> SMIDDDGYRPNVGIVICNRQGQVMWARRFGQHSWQFPQGGINPGESAEQAMYRELFEEVGLSRKDVRILASTRNWLRYKLPKRLV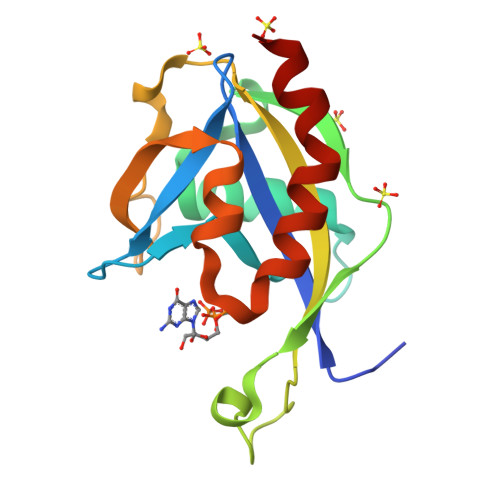RWDTKPVCIGQKQKWFLLQLVSGDAEINMQTSSTPEFDGWRWVSYWYPVRQVVSFKRDVYRRVMAAFASVVMSLQE In order to gain insight into the function and the post-translational maturation process of the glycosylated 66.3 kDa protein, three crystal structures were determined that represent different maturation states. These structures demonstrate that the 28 kDa and 40 kDa fragment which have been derived by a proteolytic cleavage remain associated. The core αββα sandwich fold and a cysteine residue at the N-terminus of the 40 kDa fragment (C249) classify the 66.3 kDa protein as a member of the structurally defined N-terminal nucleophile (Ntn) hydrolase superfamily. However, the structural classification of the 66.3 kDa protein as an Ntn hydrolase implies a hydrolytic activity on a kind of non-peptide amide bond as commonly observed for Ntn hydrolases.

The average temperature factors of only 24.1 Å2 and 19.5 Å2 for the amino acids of chains A and B, respectively, indicate an overall well defined conformation of the 66.3 kDa protein structure. The crystal structure contains seven N-acetylglucosamine moieties (NAG) in total, which are part of five N-glycans at the asparagine residues 93, 115, 236, 441 and 520 and are well defined in the electron density map. The three N-glycosylation sites of the 40 kDa fragment surround a prominent cavity – the putative substrate binding pocket – in close proximity, while the remaining two sites are localized on the opposing side of the protein molecule. Additionally, two intramolecular disulfide bridges are formed between C147 and C157 of the N- as well as between C497 and C500 of the C-terminal fragment. Non-interpreted electron density was found at the sulfhydryl group of C249, which is the N-terminal cysteine of the 40 kDa fragment. This sulfhydryl group appears to be partially oxidized which could be a consequence of the fact that the 66.3 kDa protein was purified and crystallized in the absence of a reducing agent. C249 was modeled as cysteine sulfonic acid (OCS). The oxidized side chain of this N-terminal cysteine is involved in the octahedral coordination of a cation, which is additionally bound by the side chains of S246, E328, T330 and Y379 as well as by the main chain carbonyl group of D315. Since sodium acetate was present in the crystallization buffer and due to the absence of a peak in the anomalous electron density maps calculated with diffraction data sets collected at a wavelength of 0.8 Å, 1.7 Å and 1.9 Å as well as the results of fluorescence scans (carried out at BESSY BL14.1, data not shown), it seems likely that a Na+ cation is bound to the protein. This is further supported by the octahedral coordination and metal-ligand atom distances of 2.7 – 3.1 Å.

> LPTLGPGWQRQNPDPPVSRTRSLLLDAASGQLRLEDGFHPDAVAWANLTNAIRETGWAYLDLSTNGRYNDSLQAYAAGVVEASVSEELIYMHWMNTVVNYCGPFEYEVGYCEKLKNFLEANLEWMQREMELNPDSPYWHQVRLTLLQLKGLEDSYEGRLTFPTGRFTIKPLGFLLLQISGDLEDLEPALNKTNTKPSLGSGS;> CSALIKLLPGGHDLLVAHNTWNSYQNMLRIIKKYRLQFREGPQEEYPLVAGNNLVFSSYPGTIFSGDDFYILGSGLVTLETTIGNKNPALWKYVQPQGCVLEWIRNVVANRLALDGATWADVFKRFNSGTYNNQWMIVDYKAFLPNGPSPGSRVLTILEQIPGMVVVADKTAELYKTTYWASYNIPYFETVFNASGLQALVAQYGDWFSYTKNPRAKIFQRDQSLVEDMDAMVRLMRYNDFLHDPLSLCEACNPKPNAENAISARSDLNPANGSYPFQALHQRAHGGIDVKVTSFTLAKYMSMLAASGPTWDQCPPFQWSKSPFHSMLHMGQPDLWMFSPIRVPWDGRGSHHHHHHG Fructosyl peptide oxidases (FPOX) are deglycating enzymes that find application as key enzymatic components in diabetes monitoring devices. The inability of wild type FPOXs to act on intact proteins is the most critical issue limiting both their diabetes detection efficiency and their protein deglycation potential. This is due to their buried active site and narrow access tunnel, as determined in multiple crystal structures. In that account, using a rational design approach involving a five-amino acid deletion at the entrance of the active site and a number of further mutations, we described a stable PnFPOX mutant (named L3-35A) that, relative to the wild type enzyme, features a significantly wider and shorter access tunnel.

Hence, we set out to design mutations to enhance the catalytic activity of X02A, the most thermally-stable mutant of our library. In the first design (X02B), four mutations were introduced in positions that are directly facing the tunnel in order to match the residues found in PnFPOX (D60G, A61V, D62S, D368H). In essence, by reintroducing conserved tunnel-lining residues in the X02A sequence, we generated the X02B and X02C mutants and we tested their activity toward the same panel of substrates that were tested with the parent enzyme. It is worth noting that the X02B and X02C enzymes present limited activity toward the dipeptide (≈ 0.87 and 1.62 U/mg, respectively) compared to the WT (32.60 U/mg). However, while the WT significantly shows little, if any, ability to catalyze the oxidative reaction on the F6P hexapeptide (0.78 U/mg, which is equivalent to 2.4% of the activity on fVH), the X02B and X02C mutants feature significant activity also on the hexapeptide (0.18 and 0.43 U/mg, which are equivalent to 20.7% and 26.5% of the activity observed on the fVH). The comparison shows that X02B and X02C have significantly higher activity than AnFPOX-47 toward F6P. Moreover, X02B and X02C feature a much higher Tm relative to all the other L3-35A mutants, i.e. 60.17 °C and 64.02 °C respectively. The X02B enzyme features a wide and short tunnel (bottleneck radius of 3.0 Å and length of 10.2 Å), in between the WT and its parent L3-35A, while at the same time showing a similar activity on both small and larger substrates. Hence, the wider tunnel of X02B, while reducing the stabilization of small substrates (and, as a consequence, the catalytic activity towards them) allows larger substrates to access the catalytic site more easily, leading to comparable enzymatic activity.

> MAPSRANTKVIVVGGGGTIGSSTALHLVRSGYTPSNVTVLDAYPIPSCQSAGNDLNKIMGVSADPAADAARQMWNEDELFKKFFHNTGRLDCAHGEKDIADLKKLYQNLVDWGLDATVEWLDSEDEILKRMPQLTRDQIKGWKAIFSKDGGWLAAAKAIKAIGEYLRDQGVRFGFYGAGSFKQPLLAEGVCIGVETVDGTRYYADKVVLAAGAWSPTLVELQEQCVSKAWVYGHIQLTPEEAARYKNSPVVYNGDVGFFFEPNEHGIIKVCDEFPGFTRFKMHQPFGAKAPKRISVPRSHCKHPTDTIPDASIVRIRRAIATFMPQFKNKPLFNQAMCWCTDTADGHLLICEHPEWKNFYLATGDSGHSFKLLPIIGKYVVELLEGTLADELAHKWRWRPGSGDALKSRREAPAKDLADMPGWNHDHHHHHH> MAVRLTFDGQKLTWPGIGIFKATTGLPDLQWPDKQCVPDAAIPEGNYKLFIQFQGEAPIRNAADCDLGPSWGWSTIPRGQAAGTCEIYWANWGYNRIRLESADEKTRKACGGKRGGFYIHDSTKGYSHGCIEVEPVFFRILKQETEKENGEKTF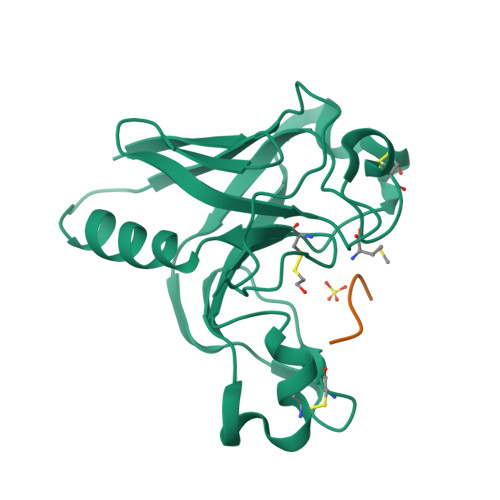TVNVKYVSGQQTNGGTKQGE;> HHHHHH6-[HYDROXY-(5,5,8,8-TETRAMETHYL-5,6,7,8-TETRAHYDRO-NAPHTALEN-2-YL)-METHYL]-NAPHTALENE-2-CARBOXYLIC 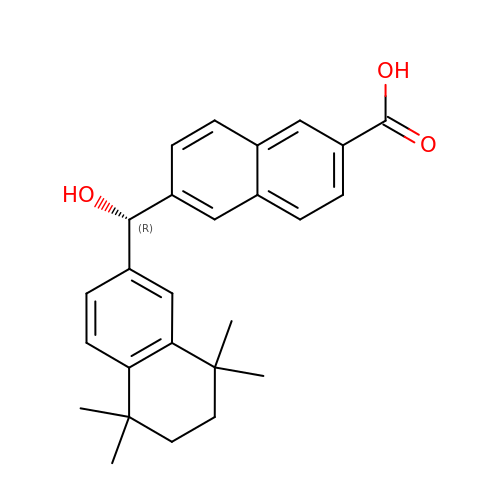ACID | C26 H28 O3 | AYAJZQYENGWICE-QHCPKHFHSA-N>LPTAQEVQGLMARYIELVDVGDIEAIVQMYADDATVEDPFGQPPIHGREQIAAFYRQGLGGGKVRACLTGPVRASHNGCGAMPFRIEMVWNGQPCAVDVISVMRFDEHGRIQTMQAY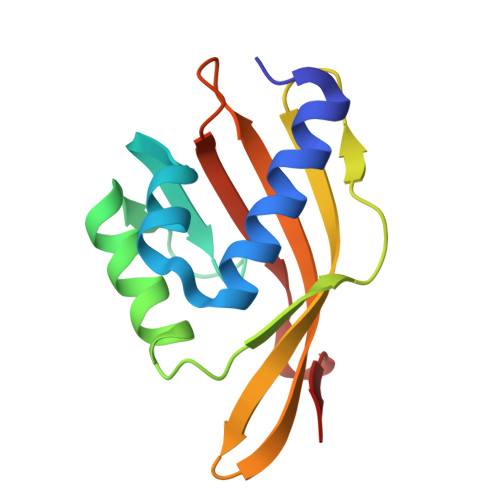WSEVNLSV[2x]> MGGSHHHHHHGMASLAPGSSRVELFKRQSSKVPFEKDGKVTERVVHSFRLPALVNVDGVMVAIADARYETSFDNSLIDTVAKYSVDDGETWETQIAIKNSRASSVSRVVDPTVIVKGNKLYVLVGSYNSSRSYWTSHGDARDWDILLAVGEVTKSTAGGKITASIKWGSPVSLKEFFPAEMEGMHTNQFLGGAGVAIVASNGNLVYPVQVTNKKKQVFSKIFYSEDEGKTWKFGKGRSAFGCSEPVALEWEGKLIINTRVDYRRRLVYESSDMGNTWLEAVGTLSRVWGPSPKSNQPGSQSSFTAVTIEGMRVMLFTHPLNFKGRWLRDRLNLWLTDNQRIYNVGQVSIGDENSAYSSVLYKDDKLYCLHEINSNEVYSLVFARLVGELRIIKSVLQSWKNWDSHLSSICTPADPAASSSERGCGPAVTTVGLVGFLSHSATKTEWEDAYRCVNASTANAERVPNGLKFAGVGGGALWPVSQQGQNQRYHFANHAFTLVASVTIHEVPKG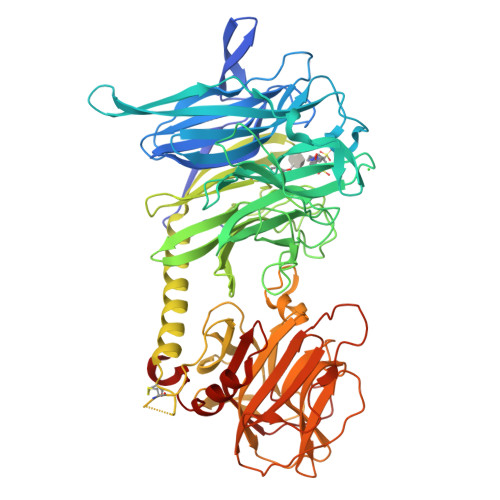ASPLLGASLDSSGGKKLLGLSYDKRHQWQPIYGSTPVTPTGSWEMGKRYHVVLTMANKIGSVYIDGEPLEGSGQTVVPDERTPDISHFYVGGYKRSGMPTDSRVTVNNVLLYNRQLNAEEIRTLFLSQDLIGTEAHMD>MVIKAKSPAGFAEKYIIESIWNGRFPPGS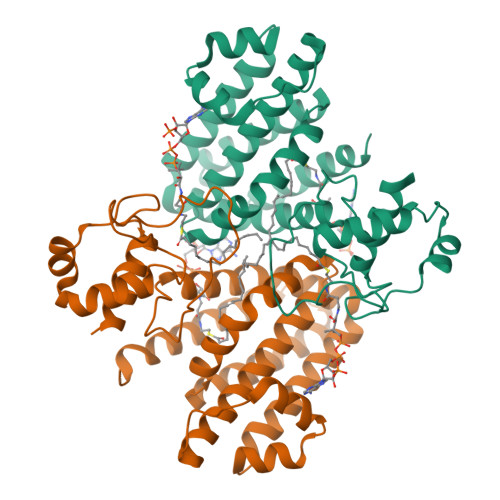ILPAERELSELIGVTRTTLREVLQRLARDGWLTIQHGKPTKVNQFMETSGLHILDTLMTLDAENATSIVEDLLAARTNISPIFMRYAFKLNKESAERIMINVIESCEALVNAPSWDAFIAASPYAEKIQQHVKEDSEKDELKRQEILIAKTFNFYDYMLFQRLAFHSGNQIYGLIFNGLKKLYDRVGSYYFSNPQARELAMEFYRQLLAVCQSGEREHLPQVIRQYGIASGHIWNQMKMTLPSNFTEDDC[2x]>[4x]MATKTSIHPSVNELYQRLAEDQLSNCFDRFDPQEKIRCNYCELGVSCQLCSNGPCRINEKVGATLGVCGINADGMAMRYMLLRNVMGTSTYTYHAYEAYKTLKMTALGNTPFTITDKDKLYQMAKDLELNTEGKPEDVAVRLSDFLIWELYRDYDEPGKMIEVYAPLKRKEVWRKLGIYPAGPLHELKDAAASCLTNVDGDYVSLATKGLRLGLSCIYGAQIGLELVQDILFGTGMPHEMDVDLGIFDADYINIVFNGHEPFVGVALILAAKEAVNQDKAKAAGAKSLRIYGSIESGQEVVQRFQKDEVFRGLTGNWLTIEPMLATGAVDVLAMDMNCSPPNLGPLAEKYGATLVSVSRLVRFPGIHHFLDYKPSEVREIAQKIIDIAVDSFKNKRHGKITPKIPANIQKAITGFTPEAILKALGGSINPLIEVIKAGKIKGAVGLINCTTLKNGPQDYVTVNLAKELIKRDILILSGGCGNHALEVAGLCNLDAINLAGPGLSEVCRNLNIPPVLSFGTCTDTGRISLVVTALANALNVDTADLPVAVTAPMYMEQKATIDALFALAYGLYTHVAPDPPVMGAPNLVKLLTRDLPSITGGRIAVGSDPVKVADDILAHINDRRAKLGI

Here, we report on the structure and reactivity of such a deviant enzyme, termed CooS‐VCh. Its structure reveals the typical CODH scaffold, but contains an iron‐sulfur‐oxo hybrid‐cluster. Although closely related to true CODHs, CooS‐VCh catalyzes neither CO oxidation, nor CO2 reduction. The active site of CooS‐VCh undergoes a redox‐dependent restructuring between a reduced [4Fe‐3S]‐cluster and an oxidized [4Fe‐2S‐S*‐2O‐2(H2O)]‐cluster.

Potential gas channels around the hybrid‐cluster were calculated for the oxidized and reduced structures of CooS‐V Ch using MOLE. Additionally, we pressurized CooS‐V Ch crystals with Xe to probe hydrophobic channels. Using the anomalous scattering contribution of Xe atoms at a wavelength of 1.90 Å, 64 Xe atoms were located in the four molecules of the asymmetric unit in which each molecule has approx. 15 Xe atoms bound (Figure S7‐A). When the four molecules with their bound Xe atoms are superimposed, common positions of Xe atoms in the interior of the structure fit well to the calculated channel.> SGAQQRELERMAEVLVTGEQLRLRLHEEKVIKDRRHHLKTYPNCFVAKELIDWLIEHKEASDRE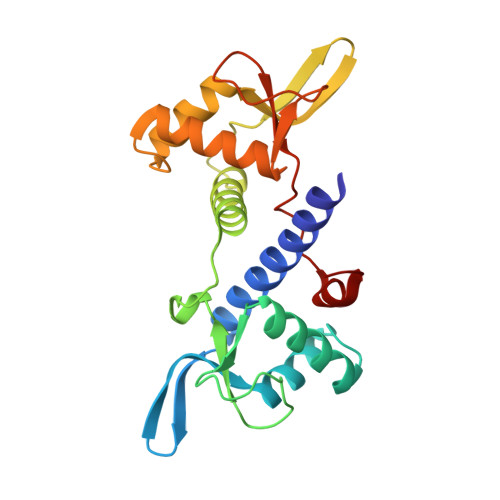TAIKLMQKLADRGIIHHVCDEHKEFKDVKLFYRFRKDDGTFPLDNEVKAFMRGQRLYEKLMSPENTLLQPREEEGVKYERTFMASEFLDWLVQEGEATTRKEAEQLCHRLMEHGIIQHVSSKHPFVDSNLLYQFRMNFRRRRRLMELLNEKS>GAMGEPPLATRATAPPGVLKIFGAGLASGANYKSVLATARSTARELVAEALERYGLAGSPGGGPGESSCVDAFALCDALGRPAAAGVGSGEWRAEHLRVLGDSERPLLVQELWRARPGWARRFELRGREEARRLEQEAFGAADSEGTGAPSWRPQK[2x];>MREYKLVVLGSGGVGKSALTVQFVQGIFVEKYDPTIEDSYRKQVEVDAQQCMLEILDTAGTEQFTAMRDLYMKNGQGFALVYSITAQSTFNDL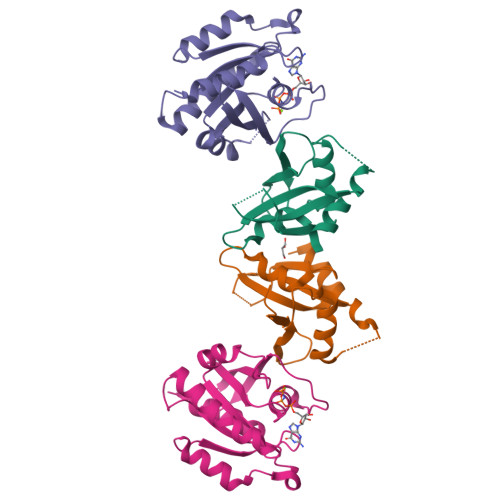QDLREQILRVKDTDDVPMILVGNKCDLEDERVVGKEQGQNLARQWNNCAFLESSAKSKINVNEIFYDLVRQINR[2x]>[2x]LPDSVDWREKGCVTEVKYQGSCGACWAFSAVGALEAQLKLKTGKLVTLSAQNLVDCSTEKYGNKGCNGGFMTTAFQYIIDNKGIDSDASYPYKAMDQKCQYD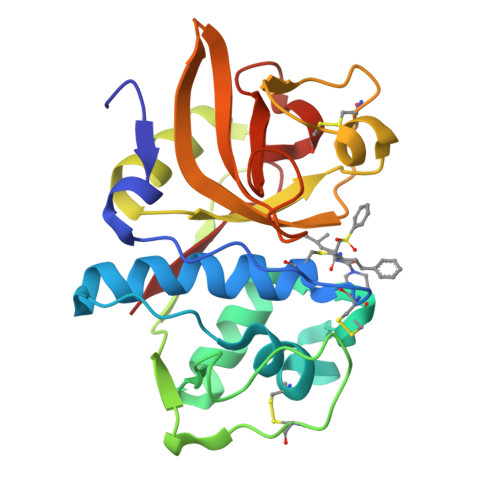SKYRAATCSKYTELPYGREDVLKEAVANKGPVSVGVDARHPSFFLYRSGVYYEPSCTQNVNHGVLVVGYGDLNGKEYWLVKNSWGHNFGEEGYIRMARNKGNHCGIASFPSYPEI> GPLGSMENSCNFNNSIKNVIVFYINEKALIEEKKMLSCYENKLLNLIKEDCENIMLKYKPNLSYICSLLKVDDTSEENIKHIKDQIIESLENDNRPSVKLAIISLISMIVEMNGYKGKNIPMSFLIEDIALKISE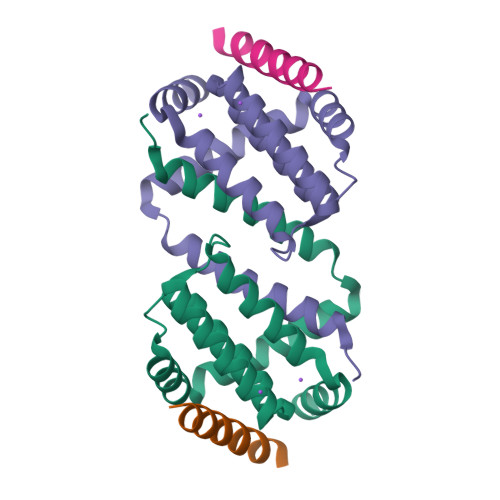NSEDLINFINIKNKQKS;> VPQDASTKKLSECLKRIGDELDSNMELQ> GASCDSFNEDLPECRLSVKFKYDYNMEFADAFHAQVDKVELYVFDKNGKYLFKQAEEGSALSTGNYLMEVELPVGQYQFMAWAGARDSYDITSLTPGVSTLTDLKLKLKREASLIINKRMETLWYGEVINVNFDGTVHQTETINLIRDTKIVRFGFQSYTGSWTLDMNDYDYEIIESNGHLGHDNSLLDDDVLSFRPYYMEQKDPATAY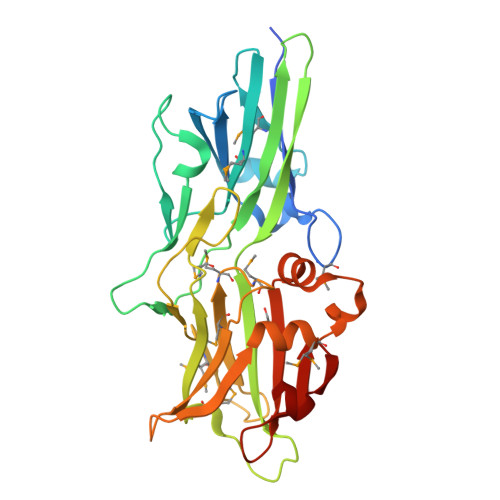VDMNTMRLMEDRKTRLVLTEKASGKRVFDINLIDYLAMTNAEGKNLSTQEYLDRQSNYHIIFFLSESWLAVQIVVNGWVHRIQEENQ>[2x]ARNIKEVLESAMDLITENQRKGSLEVTGIPTGFVQLDNYTSGFNKGSLVIIGARP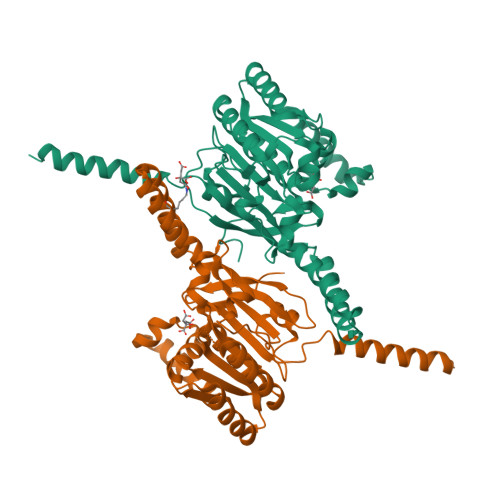SMGKTSLMMNMVLSALNDDRGVAVFSLEMSAEQLALRALSDLTSINMHDLESGRLDDDQWENLAKCFDHLSQKKLFFYDKSYVRIEQIRLQLRKLKSQHKELGIAFIDYLQLMSGSKATKERHEQIAEISRELKTLARELEIPIIALVQLNRSLENRDDKRPILSDIKDSGGIEQDADIVLFLYRGYIYQMRAEDNKIDKLKKEGKIEEAQELYLKVNEERRIHKQNGSIEEAEIIVAKNRNGATGTVYTRFNAPFTRYEDMPIDSHLEEGQETKVDYDIVTT>MSGGGVFTDILAAAGRIFEVMVEGHWETVGMLFDSLGKGTMRINRNAYGSMGGGSLRGS[14x]

Detailed structural information is available for representatives of many light-harvesting antenna systems, but not for the proteinaceous baseplate of chlorosomes. This structure has three essential functions: (i) ensuring the structural integrity of the chlorosome organelle, (ii) connecting the chlorosomes to the photosynthetic reaction centre in the cell membrane and (iii) transferring excitation energy from the protein-free BChl c/d/e antennae towards the reaction centre. Previous studies have shown that roughly 1,000–2,000 of CsmA protein subunits, each binding one BChl a pigment molecule, constitute the baseplate. The baseplate is oriented towards the cytoplasmic membrane and in the Cba. tepidum attaches to the so-called Fenna-Matthews-Olson (FMO) protein complex, which is the last antenna before the energy reaches the reaction centre.

The novel approach in the present work to structural studies of the baseplate became possible with a bchK mutant of Cba. tepidum that forms modified chlorosomes, termed carotenosomes, with a fully functional baseplate formed by CsmA protein and BChl a pigment but lacking self-assembled BChl c antenna elements. Hence, by combining all types of experimental constraints: local high-resolution structural information from solid-state NMR, orientation between BChl a pigments from isotropic and anisotropic CD, LD, ab initio calculations, and global structural information from cryo-EM, together with the symmetry information, it was possible to derive a unique and precise structure for the CsmA-BChl a baseplate. CD spectra analysis and ab initio calculations demonstrate that the basic building block of the baseplate structure is a symmetric CsmA dimer, which is translated along two perpendicular directions to form a two-dimensional lattice structure. In accord with indications from earlier studies, the CsmA monomers form helical structures with a slight curvature. The data presented here reveal that the helices form rods by head-to-tail translational association in a tight interface allowed by the small amino acids of in particular G15, G39 and A12 flanked by other relatively small polar amino acids such as T8, S35 and N46. The helices are amphipathic leading to formation of a hydrophobic and a hydrophilic interface. The hydrophilic interface pairs the side of the helices with electrostatic interactions through oppositely charged side-chains. The hydrophobic interface is further stabilized by symmetry-related packing of aromatic rings of F7/F7* and F18/F18* and clustering of other hydrophobic residues. The BChl a ligand coordinates to the side-chain of H25 and form pairs, which are almost co-planar orthogonal to the plane of the baseplate and with the centres separated by ca. 15 Å along the rod axis.>[2x]MAHHHHHHMIDPNSLLPKLPSPDELKPFPTVQQTIFRGHEGRVRSVAIDPTGVALATGGDDGTVRVWELLTGRQVWSVKLNGDEAVNTVRWRPTKDTFILAAAAGEDIFLMIPTHPSVTPALDQASRDILNAGFGHATNGKQQANLPPGKEPPGKWARPGTRLEDEGVLLRITVRSTIKAISWHRRGDHFATVSPSGQRSSVAIHTLSKHLTQIPFRKLNGLAQTASFHPLRPLFFVATQRSIRCYDLQKLELVKIVQPGAKWISSFDVHPGGDNLVVGSYDKRLLWHDLDLSNRPYKTMRFHTEAIRAVRFHKGGLPLFADAS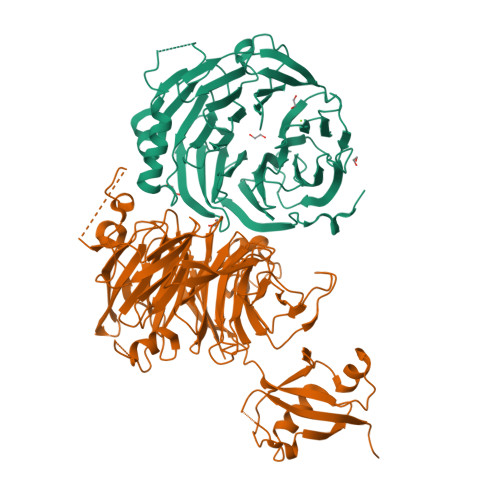DDGSLQIFHGKVPNDQLENPTIVPVKMLKGHKVVNKLGVLDIDWHPREPWCVSAGADGTARLWM;>[2x]GGAHMDAPMEDAPAPVAQVKVIFTTTEPDLELPESKRQLLVPADIRRYGLSRILNSESMLDTGSIPFDFLINGSFLRSSLEDYLTSNGLSLETTLTLQYVRSLIPPVYEASFEHDDWVSAVDVLSATSPAGRWSSAANSSAAVQPGQERVLSASYDGLLRIWNASGSVIATSPSGSHGGHTASIKAAKFLTSDRLASAGMDRTVRVWKYTESDHFTGELKPTLELYGHTGSVDWLDVDGHSKHILTASADGAIGFWSASKASAPEPDASLLPGAHVSKRRKATSSVSTAQRGPLGLWSIHTAPATAAIFDPRDRTVAYSASQDHTVRTLDLTTGQVVSTLTLTHPLLSLSALTRAGTTSPLLAAGTSARHITMVDPRASSATTSVMTLRGHANKVVSLSPSPENEYSLVSGSHDGTCRVWDLRSVRPATKEEGSLGGVSEPVYVIERESWASKGKKKRPVAGDGCKVFSVVWDKLGIFSGGEDKKVQVNRGRNIVTEQK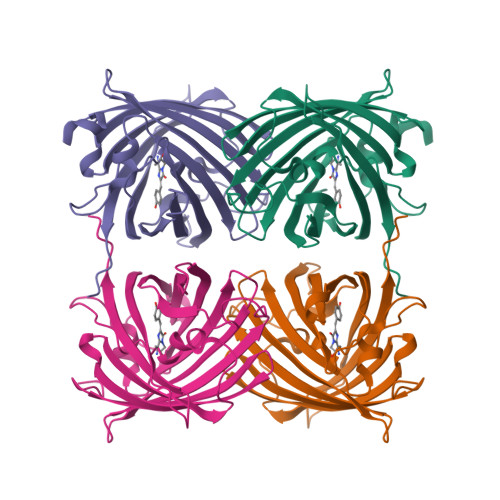>[2x]GSHMMALSKHGLTKDMTMKYRMEGCVDGHKFVITGHGNGSPFEGKQTINLCVVEGGPLPFSEDILSAVFDYGNRVFTDYPQGMVDFFKNSCPAGYTWQRSLLFEDGAVCTASADITVSVEENCFYHESKFHGVNFPADGPVMKKMTINWEPCCEKIIPVPRQGILKGDVAMYLLLKDGGRYRCQFDTVYKAKTDSKKMPEWHFIQHKLTREDRSDAKNQKWQLAEHSVASRSALA> GGDDDDTGYLPPSQAIQDALKKLYPNATAIKWEQKGVYYVADCQADGREKEVWFDANANWLMTETELNSINNLPPAVLTAF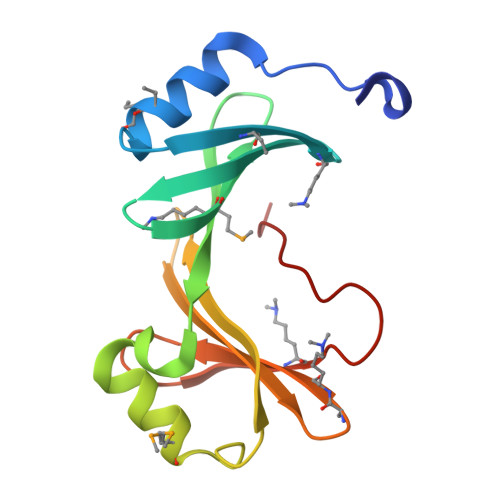MESSYNNWVVDDVVILEYPNEPSTEFVVTVEQGKKVDLYFSEGGGLLHEKDVTNGDDTHWPRV> FACKTANGTAIPIGGGSANVYVNLAPVVNVGQNLVVDLSTQIFCHNDYPETITDYVTLQRGAAYGGVLSSFSGTVKYNGSSYPFPTTSETPRVVYNSRTDKPWPVALYLTPVSSAGGVAIKAGSLIAVLILRQTNNYNSDDFQFVWNIYANNDV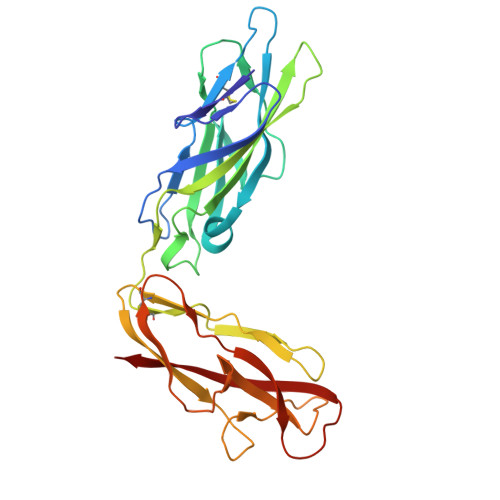VVPTGGCDASARDVTVTLPDYPGSVPIPLTVYCAKSQNLGYYLSGTTADAGNSIFTNTASFSPAQGVGVQLTRNGTIIPANNTVSLGAVGTSAVSLGLTANYARTGGQVTAGNVQSIIGVTFVYQ>[2x]GGEGIQPSKKLITRDYKVKEFNKIDAGTVGNIYYTQSTDGKTDLQIYGPDNIVALIQVAVKDNTLFLSIDKSKKVRNFKKMKITITSPTLNGISFKGVGDVHIENGLTT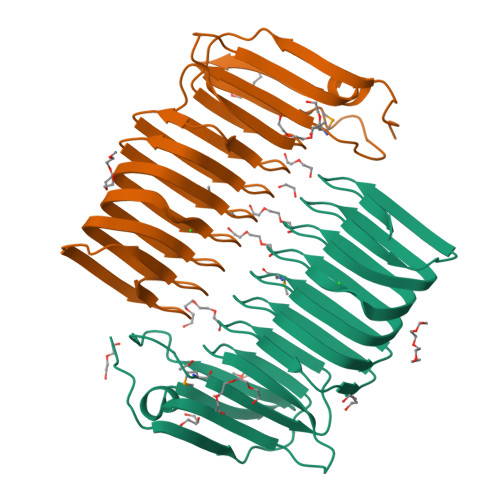DNLDIESKGVGNVDIQSLTCQKLNVQSMGVGDVKLEGTAQIAALHSKGVGNIEAGNLRANAVEASSQGVGDITCNATESIDAAVRGVGSIKYKGSPTIKSLSKKGVGTIKNI>GPAMASKSPSEEVYPVKAFGLAAKDSSGLFSPFNFSRRATGEHDVQLKVLYCGTCQYDREMSKNKFGFTSYPYVLGHEIVGEVTEVGSKVQKFKVGDKVGVASIIETCGKCEMCTNEVENYCPEAGSIDSNYGACSNIAVINENFVIRWPENLPLDSGVPLLCAGITAYSPMKRYGLDKPGKRIGIAGLGGLGHVALRFAKAFGAKVTVISSSLKKKREAFEKFGADSFLVSSNPEEMQGAAGTLDGIIDTIPGNHSLEPLLALLKPLGKLIILGAPEMPFEVPAPSLLMGGKVMAASTAGSMKEIQEMIEFAAEHNIVADVEVISIDYVNTA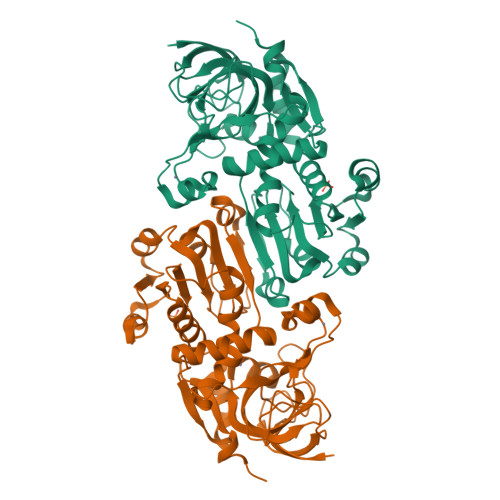MERLDNSDVRYRFVIDIGNTLKSN[2x]> PDQFRAIIESPEGAGHVGYQYRRNTGSTMRMVSDVLDERVSLWDFHCDPSGNVIQPGPNVDSRQYLQAAIDYVSSNGGGTITIPAGYTWYLGSYGVGGIAGHSGIIQLRSNVNLNIEGRIHLSPFFDLKPFQVFVGFDNGDPASSGNLENCHIYGHGVVDFGGYEFGASSQLRNGVAFGRSYNCSVTGITFQNGDVTWAITLGWNGYGSNCYVRKCRFINLVNSSVNANHSTVYVNCPYSGVESCYFSMSSSFARNIACSVQLHQHDTFYRGSTVNGYCRGAYVVMHAAEAAGAGSYAYNMQVENNIAVIYGQFVILGSDVTATVSGHLNDVIVSGNIVSIGERAAFSAPFG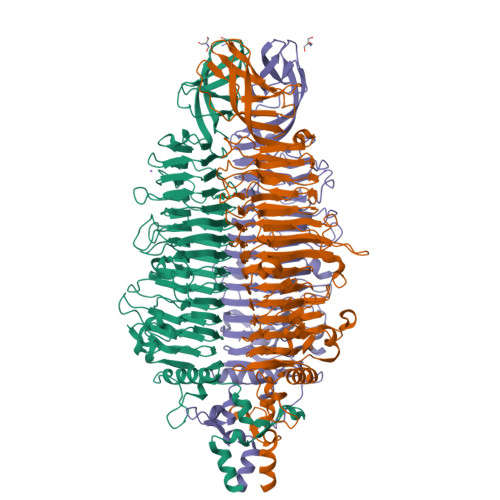AFIDIGPDNSGASNVQDIQRVLVTGNSFYAPANITDSAAITLRANLNGCTFIANNFDCRYMVYNAPGTTSPVVQNLVWDKSNVIGGTHANQRAGQNLFDMQFASVVNSTIEVQLSCEDLSMFSCILFPASCQLSYSKITVDSAWTKSMSNTAVFEGNQQAGANVYVSYPATVNLTSYNTQGAVPFFSTDTNYAWVTSAYSLSINENLDFSPPATYTNKANGQLVGVGYNEIGGVRSVSVRLMLQRQV2,2'-[heptane-1,7-diylbis(oxybenzene-4,1-diyl)]bis(1H-imidazole) | C25 H28 N4 O2 | 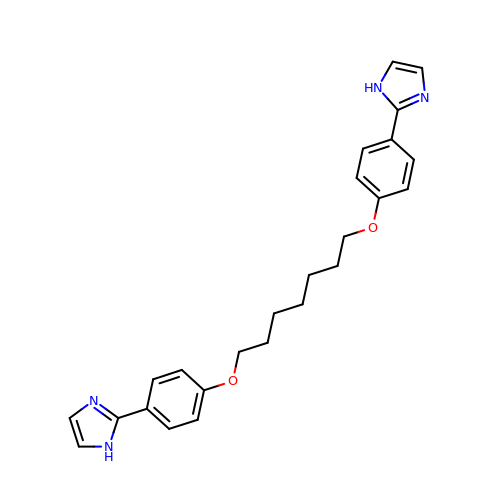LGLZBONOWHSGOF-UHFFFAOYSA-N In this context, the plant caseinolytic protease (Clp) complex plays an important role in degradation of accumulated and misfolded proteins in chloroplasts wherein the chaperones aid in ATP-dependent unfolding of protein substrates to be degraded by the associated protease machinery. The structured, mature forms of AtClpC1/C2/D consist of three distinct domains such as a short N-terminal domain (NTD) and two ATPase domains, a feature very similar to bacterial ClpC proteins. The N-terminal domain of ClpC1 is known to perform the regulatory function of substrate recognition, either directly or indirectly through the adaptor proteins ClpS1/ClpF for which it becomes a binding platform161718, whereas no adaptor proteins have so far been reported for ClpD. Here we report and analyse the crystal structures of AtClpC1 residues 94 to 238 and AtClpD residues 79 to 233 (hereafter mentioned as AtClpC1 NTD and AtClpD NTD respectively) that correspond to the ClpC NTD of eubacteria.

The 1.20 Å structure showed AtClpC1 N-terminal domain (residues 94–238) to be a α-helical domain, having 66% helical content and made up of eight tightly packed α-helices: α1 (E100-L116), α2 (T123-E133), α3 (I137-M145), α4 (L149-I160), α5 (P175-L191), α6 (S198-E208), α7 (V212-L220) and α8 (P224-N238). The two central helices: α2 and α6 which are rich in the hydrophobic residues Leu and Ile contribute significantly to the packing. The fold of AtClpC1 NTD contains two repeats of a 4-helix motif that share 46% sequence identity and 84.1% similarity in a region of 63-residue overlap. A 14-residue long loop between α4 and α5 connects the two repeats. The two halves that stay in close proximity are related by a pseudo two-fold axis of symmetry. Strong sequence identity and conservation of secondary structure between the two halves suggest the possibility of an early evolutionary gene duplication event that could have resulted in this repeated motif, as has been predicted for the N-terminal domain of bacterial ClpA and other ClpC proteins. A query to the DALI database and PDBeFold server with AtClpC1 NTD structure coordinates yielded NTD of mycobacterial ClpC1 and other Gram-positive bacterial ClpC as the most similar structures. A comparison of the crystal structures of MtClpC1-CymA complex and AtClpC1 shows the CymA-interacting residues to be conserved. Phe95, Phe173, Lys178 and Glu182 of AtClpC1 occupy the same position as the residues involved in MtClpC1 NTD interaction with CymA. So we presume CymA would bind readily to AtClpC1 NTD as well.

> MFERFTEKAIKVIMLAQEEARRLGHNFVGTEQILLGLIGEGTGIAAKVLKSMGINLKDARVEVEKIIGRGSGFVAVEIPFTPRAKRVLELSLEEARQLGHNYIGSEHLLLGLLREGEGVAARVLENLGADPSNIRTQVIRMVGENLEHHHHHH>[93x]AEIGGDHGYNATNIAAGQTSGAVTQIGPA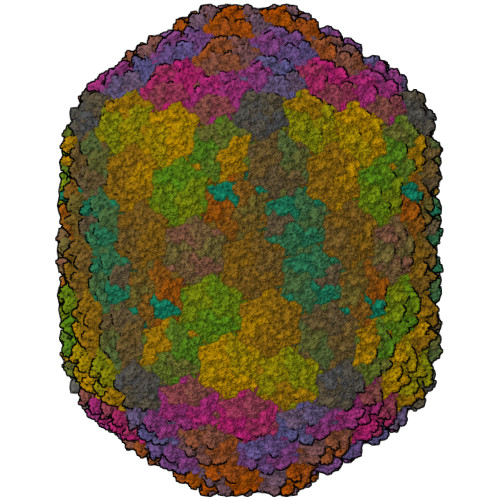VMGMVRRAIPNLIAFDICGVQPMNSPTGQVFALRAVYGKDPVAAGAKEAFHPMYGPDAMFSGQGAAKKFPALAASTQTTVGDIYTHFFQETGTVYLQASVQVTIDAGDEDEDEDEDATDAAKLDAEIKKQMEAGALVEIAEGMATSIAELQEGFNGSTDNPWNEMGFRIDKQVIEAKSRQLKAAYSIELAQDLRAVHGMDADAELSGILATEIMLEINREVVDWINYSAQVGKSGMTLTPGSKAGVFDFQDPIDIRGARWAGESFKALLFQIDKEAVEIARQTGRGEGNFIIASRNVVNVLASVDTGISYAAQGLATGFSTDTTKSVFAGVLGGKYRVYIDQYAKQDYFTVGYKGPNEMDAGIYYAPYVALTPLRGSDPKNFQPVMGFKTRYGIGINPFAESAAQAPASRIQSGMPSILNSLGKNAYFRRVYVKGI;>[5x]STTTNSNSIGRPNLVALTRATTKLIYSDIVATQRTNQPVAAFYGIKYLNPDNEFTFKTGATYAGEAGYVDREQITELTEESKLTLNKGDLFKYNNIVYKVLEDTPFATIEESDLELALQIAIVLLKVRLFSDAASTSKFESSDSEIADARFQINKWQTAVKSRKLKTGITVELAQDLEANGFDAPNFLEDLLATEMADEINKDILQSLITVSKRYKVTGITDSGFIDLSYASAPEAGRSLYRMVCEMVSHIQKESTYTATFCVASARAAAILAASGWLKHKPEDDKYLSQNAYGFLANGLPLYCDTNSPLDYVIVGVVENIGEKEIVGSIFYAPYTEGLDLDDPEHVGAFKVVVDPESLQPSIGLLVRYALSANPYTVAKDEKEARIIDGGDMDKMAGRSDLSVLLGVKLPKIII> MQSAISISKLQDVLIASVQVDLTEST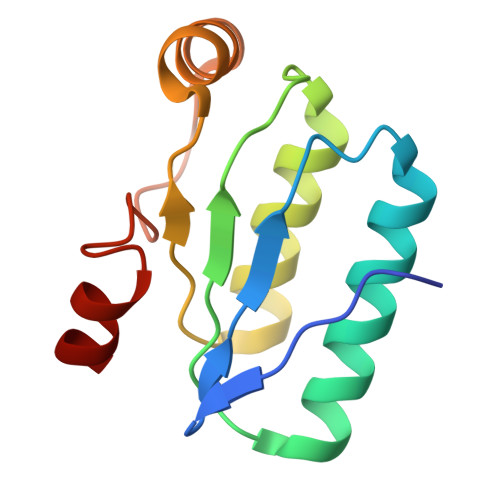LRDFSLDLLDAVKSTRAKGVMIELSGVKTLDGESMHSLLDVVKTVEVMGRRCLLVGLRPGVVIGLMDIGIDLASTLCVADLEQGFLYLE(2R)-2-[3-ISOBUTYL-2,5-DIOXO-4-(QUINOLIN-3-YLMETHYL)-1,4-DIAZEPAN-1-YL]-N-METHYL-3-(2-NAPHTHYL)PROPANAMIDE 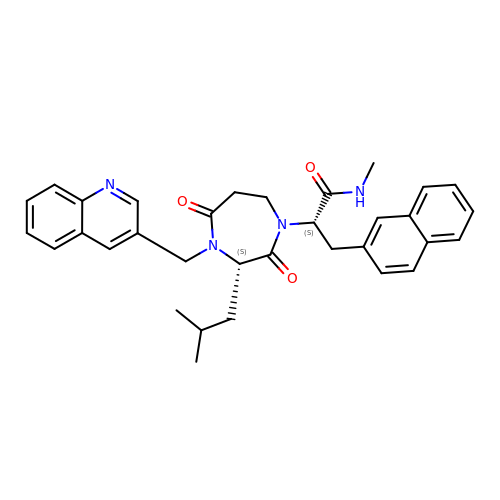| C33 H36 N4 O3 | COVPLULNDBDXTN-KYJUHHDHSA-N>LSGAIVALILVIAGVIIAIAVVLFAFGLIPGISNQGSIQVLGSGTITNSTASGSSRTIYNITITVKNTGTTSISVTSININGQPFNINGTAPSIPAGRTQPITFEVTPASGKPNFSPGASYTATIYFSNGQGAPATLIYQG[30x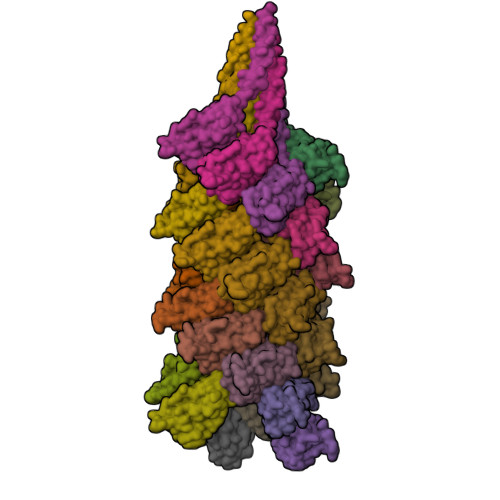]> MDPTPVSVSGGTIHFEGKLVNAACAVSTKSADQTVTLGQYRTASFTAIGDTTAQVPFSIVLNDCDPKVAATAAVAFSGQADNTNTNLLAVSSADNSTTATGVGIEILDNT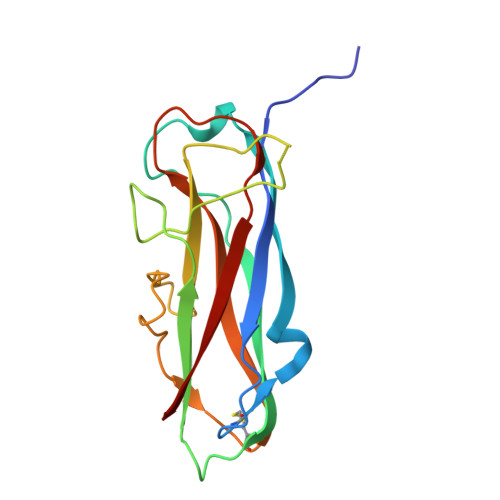SSPLKPDGATFSAKQALVEGTNTLRFTARYKATAAATTPGQANADATFIMKYE> NAINPRLTPWTYRNTSFSSLPLTGENPGAWALVRDNSAKGITAGSGSQQTTYDPTRTEAALTASTTFALRRYDLAGRALYDLDFSKLNPQTPTRDQTGQITFNPFGGFGLSGAAPQQWNEVKNKVPVEVAQDPSNPYRFAVLLVPRSVVYYEQLQRGLGLPQQRTESGQNTSTTGAMFGLKVKNAEADTAKSNEKLQGAEATGSSTTSGSGQSTQRGGSSGDTKVKALKIEVKKKSDSEDNGQLQLEKNDLANAPIKRSEESGQSV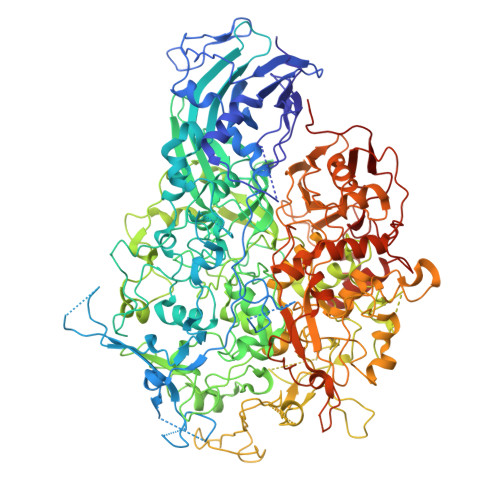QLKADDFGTALSSSGSGGNSNPGSPTPWRPWLATEQIHKDLPKWSASILILYDAPYARNRTAIDRVDHLDPKAMTANYPPSWRTPKWNHHGLWDWKARDVLLQTTGFFNPRRHPEWFDGGQTVADNEKTGFDVDNSENTKQGFQKEADSDKSAPIALPFEAYFANIGNLTWFGQALLVFGGNGHVTKSAHTAPLSIGVFRVRYNATGTSATVTGWPYALLFSGMVNKQTDGLKDLPFNNNRWFEYVPRMAVAGAKFVGRELVLAGTITMGDTATVPRLLYDELESNLNLVAQGQGLLREDLQLFTPYGWANRPDLPIGAWSSSSSSSHNAPYYFHNNPDWQDRPIQNVVDAFIKPWEDKNGKDDAKYIYPYRYSGMWAWQVYNWSNKLTDQPLSADFVNENAYQPNSLFAAILNPELLAALPDKVKYGKENEFAANEYERFNQKLTVAPTQGTNWSHFSPTLSRFSTGFNLVGSVLDQVLDYVPWIGNGYRYGNNHRGVDDITAPQTSAGSSSGISTNTSGSRSFLPTFSNIGVGLKANVQATLGGSQTMITGGSPRRTLDQANLQLWTGAGWRNDKASSGQSDENHTKFTSATGMDQQGQSGTSAGNPDSLKQDNISKSGDSLTTQDGNAIDQQEATNYTNLPPNLTPTADWPNALSFTNKNNAQRAQLFLRGLLGSIPVLVNRSGSDSNKFQATDQKWSYTDLHSDQTKLNLPAYGEVNGLLNPALVETYFGNTRAGGSGSNTTSSPGIGFKIPEQNNDSKATLITPGLAWTPQDVGNLVVSGTTVSFQLGGWLVTFTDFVKPRAGYLGLQLTGLDASDATQRALIWAPRPWAAFRGSWVNRLGRVESVWDLKGVWADQAQSDSQGSTTTATRNALPEHPNALAFQVSVVEASAYKPNTSSGQTQSTNSSPYLHLVKPKKVTQSDKLDDDLKNLLDPNQVRTKLRQSFGTDHSTQPQPQSLKTTTPVFGTSSGNLSSVLSGGGAGGGSSGSGQSGVDLSPVEKVSGWLVGQLPSTSDGNTSSTNNLAPNTNTGNDVVGVGRLSESNAAKMNDDVDGIVRT>MSEPTIYEQIGGEATFRRIVDIFYAR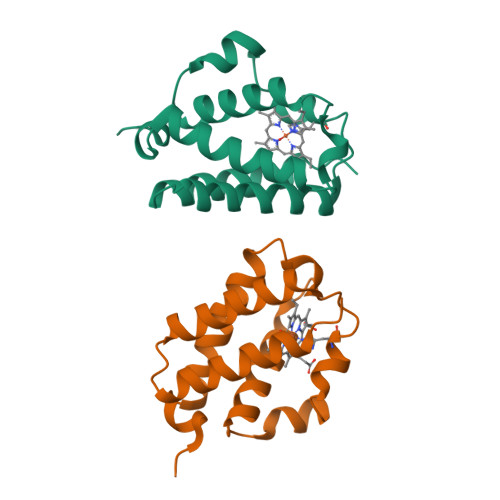VEADPRLRHLFPADLEPGKEHQRLFLMQYFGGPRTYSERRGHPRLRMRHAPFPIGPRERDAWLEHMLAALNEAGVPEPARSVMENYFRHAAQAMMNRLGED[2x]N-[2-(dimethylamino)ethyl]-3-[6-(thiophen-2-yl)imidazo[1,2-b]pyridazin-3-yl]benzamide 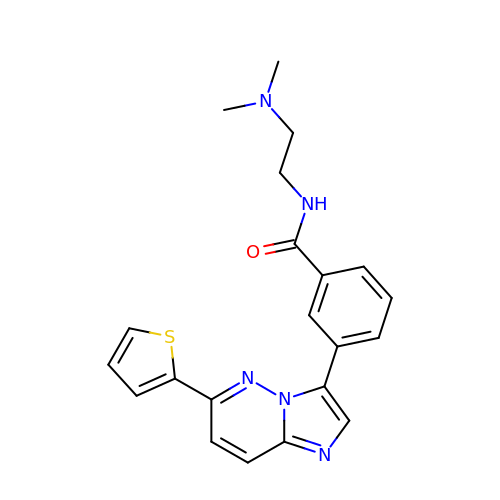| C21 H21 N5 O S | WWJQERVKTFKCOB-UHFFFAOYSA-N> AVPFVEDWDLVQTLGEGAYGEVQLAVNRVTEEAVAVKIVDMKRAVDCPENIKKEICINKMLNHENVVKFYGHRREGNIQYLFLEYCSGGELFDRIEPDIGMPEPDAQRFFHQLMAGVVYLHGIGITHRDIKPENLLLDERDNLKISDFGLATVFRYNNRERLLNKMCGTLPYVAPELLKRREFHAEPVDVWSCGIVLTAMLAGELPWDQPSDSCQEYSDWKEKKTYLNPWKKIDSAPLALLHKILVENPSAR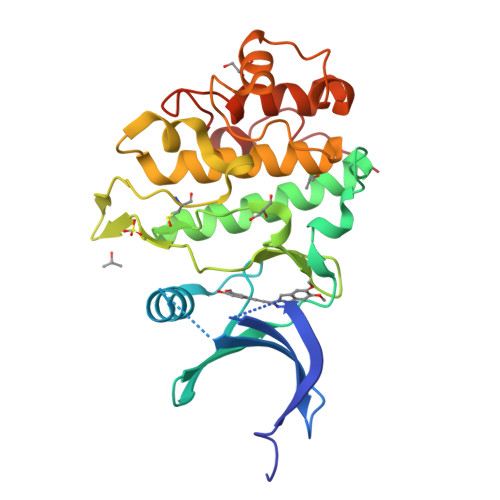ITIPDIKKDRWYNKPLK> MTQFNITWEEQLQALSKLDGLHHPHKLEDISVHWVFNPVDISVFVTCATMSSHNTHYTFKPQSSPDDAMVR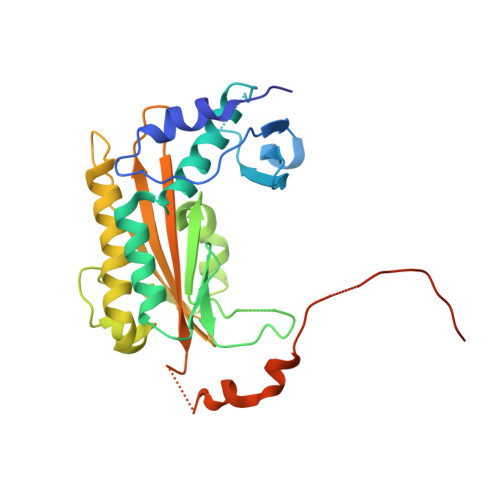EYVLSRIIADNLKYVDNLYLAAGAVICGNDEYISDGNVVGIHIADGVGGNKLILPVIEFMPGVHVDDISDKLIKSSSYQGIFKTDNLEEFEFLVDKKNANNVKELILAYTDYFANKLAFKDPAEPAVEMYQFIDRTEVYFSFEGCHPDVEEVLFTIKIVRYNQPLNSTAMQVFLKNPLLSHIRTVVRQDLPAKFVGGVLFNFKGHHHHHH> MVEDLLEHAKDILGYQRPVKVRIRPLKMSIARVSFKYGTITLDPAVLNLEEEEMFYILIHELAHLKAE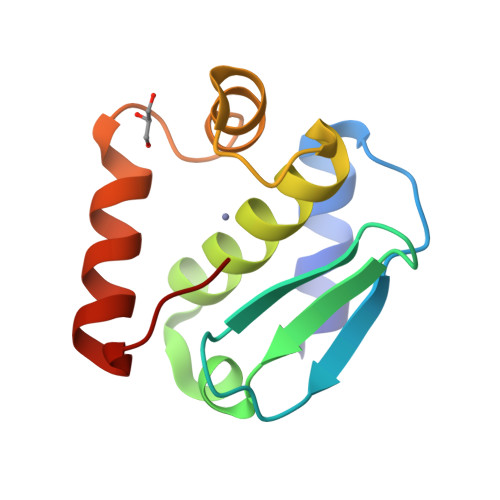TSYHSSSFWREVEKVFPGERAKEIEDRIMTKLQRNMV(5R)-6-(5-chloropyridin-2-yl)-7-oxo-6,7-dihydro-5H-pyrrolo[3,4-b]pyrazin-5-yl 4-methylpiperazine-1-carboxylate 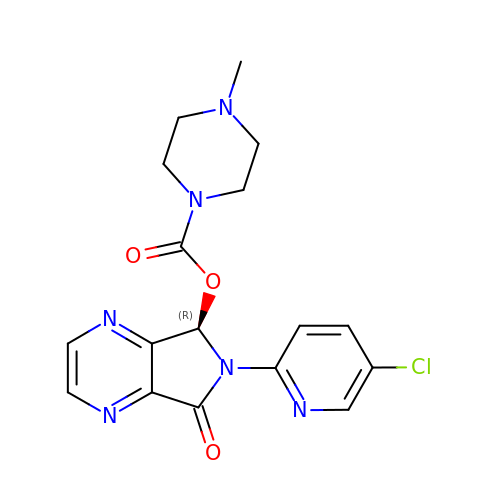| C17 H17 Cl N6 O3 | GBBSUAFBMRNDJC-MRXNPFEDSA-N>MAHHHHHHVDDDDKMAP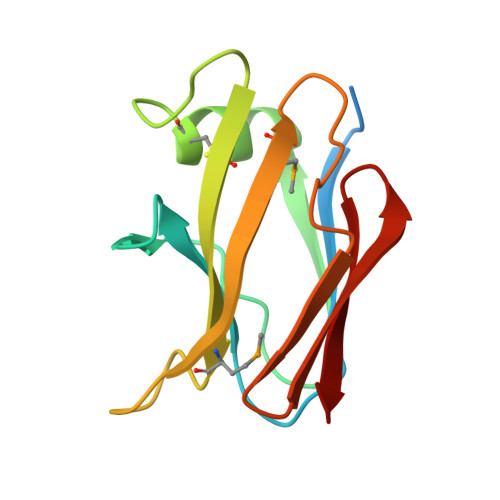AYLTTHNRTGEESNAYIAGSIPSLYPTAAYSTNQVYWNLVRLACYGHTTNGQCPALIKMATNTANPIDIGYVTMDLNTGDITPKTLSAKGYSLRVIGPGEAEITKN[2x]>MVLYFIGLGLYDERDITVKGLEIAKKCDYVFAEFYTSLMAGTTLGRIQKLIGKEIRVLSREDVELNFENIVLPLAKENEVAFLTPGDPLVATTHAELRIRAKRAGVESYVIHAPSIYSAVGITGLHIYKFGKSATVAYPEGNWFPTSYYDVIKENAERGLHTLLFLDIKAEKRMYMTANEAMELLLKVEDMKKGGVFTDDTLVVVLARAGSLNPTIRAGYVKDLIREDFGDPPHILIVPGKLHIVEA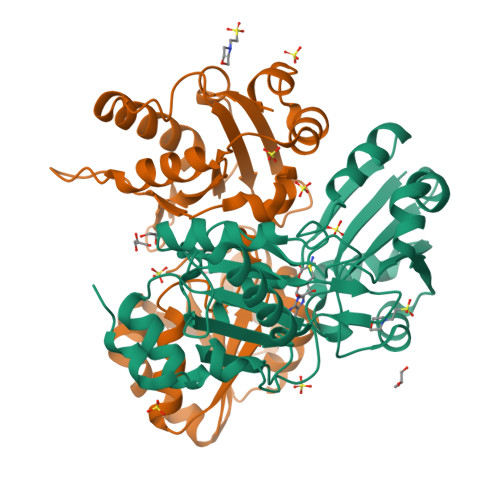EYLVEIAGAPREILRVNV[2x]> GSKPV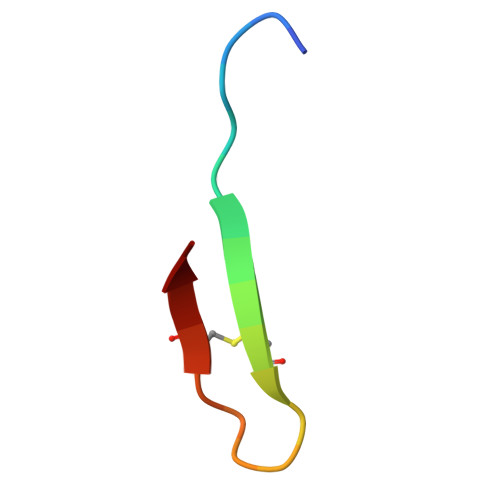PIIACNRKTGKCTRI(2R)-1-(3,8-dihydrodibenzo[b,f]pyrrolo[3,4-d]azepin-2(1H)-yl)propan-2-ol | C19 H20 N2 O | 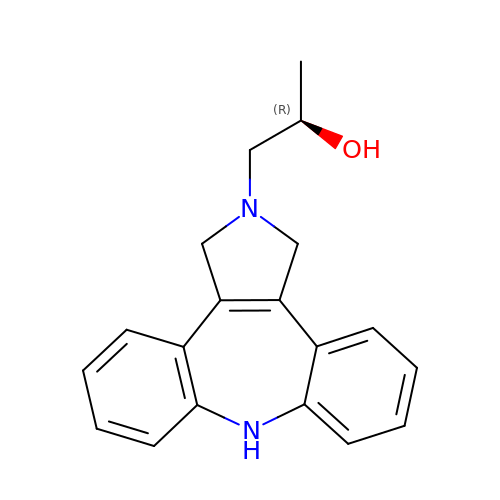KUHCFTHIRUPZQC-CYBMUJFWSA-N> MIFPKQYPIINFTTAGATVQSYTNFIRAVRGRLTTGADVRHEIPVLPNRVGLPINQRFILVELSNHAELSVTLALDVTNAYVVGYRAGNSAYFFHPDNQEDAEAITHLFTDVQNRYTFAFGGNYDRLEQLAGNLRENIELGNGPLEEAISALYYYSTGGTQLP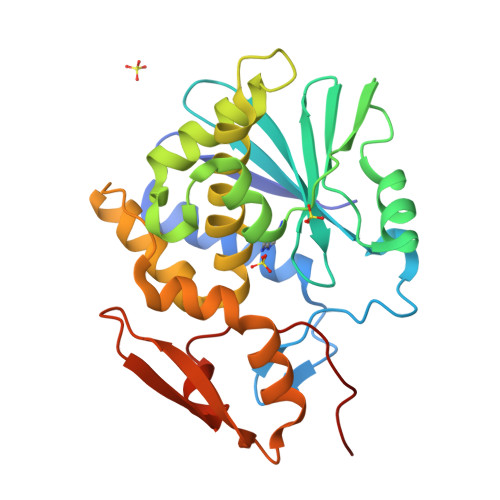TLARSFIICIQMISEAARFQYIEGEMRTRIRYNRRSAPDPSVITLENSWGRLSTAIQESNQGAFASPIQLQRRNGSKFSVYDVSILIPIIALMVYRCAPPPSSQF The ribonuclease RNase J is a key enzyme in RNA turnover and precursor processing in the model Gram-positive bacterium Bacillus subtilis and numerous other bacterial and archaeal species (1–9). Thus, in addition to the eponymous β-lactamase fold, RNase J bears C-terminal and β-CASP domains. RNase J can cleave mRNA by either endonucleolytic or exonucleolytic mode, with preference depending on the 5′ end of the RNA.

The structure reveals a homotetrameric quaternary organization that unexpectedly carries intact nucleotides of RNA at each of the active sites. This pre-cleavage structure, solved at 2.27 Å resolution, provides details of the interactions of the RNA with the catalytic site, including a network of water molecules which may facilitate acid-base chemistry. In the course of preparing the recombinant S. coelicolor RNase J, RNA originating from the E. coli expression host was found to co-purify with the enzyme. The RNA was also sequenced and identified as 5′ pCGCCU, but the remaining 3′ nucleotides could not be identified unambiguously. The 5-nucleotide sequence fitted well into the experimental electron density in the substrate-binding tunnel that encompasses the active site, but the electron density was not clearly defined for the remaining nucleotides to the 3′ end of the experimentally identified pCGCCU sequence. The RNA interacts with both the metals through the O1 and O2 oxygens of the penultimate phosphate of the 5′ terminus. The water forms a close contact to the phosphate ester oxygen (2.7 Å). It was unexpected that the RNA would be found in the catalytic site adjacent to a water molecule that is apparently ‘activated’ by Zn binding, and yet not be cleaved. The reason that the S. coelicolor RNase J/RNA complex is stalled appears to be related to the presence of 1.33 mM EDTA in the crystallization condition, because we observe that EDTA inhibits the activity of the enzyme in this concentration range. Close inspection of the active site shows that the scissile phosphate is not properly aligned with the potentially attacking water molecule to permit a bimolecular nucleophilic (SN2) attack.

>MSHPHPELGRPPALPKGGLRVTPLGGLGEIGRNMTVFEYGGRLLIVDCGVLFPEEEQPGIDLILPDFTSIRDRLDDIEGIVLTHGHEDHIGGVPFLLREKPDIPLIGSKLTLALIEAKLQEHRIRPYTLEVAEGHRERVGPFDCEFVAVNHSIPDALAVAIRTPAGMVVHTGDFKMDQLPLDGRLTDLHAFARLSEEGIDLLLADSTNAEVPGFVPPERDISNVLRQVFANARKRIIVASFASHVHRIQQILDAAHEYGRRVAFVGRSMVRNMGIARDLGYLKVPPGLVVDVKTLDDLPDSEVVLVCTGSQGEPMAALSRMANRDHQIRIVNGDTVILASSLIPGNENAVYRVINGLTRWGANVVHKGNAKVHVSGHASAGELLYFYNICRPKNLMPVHGEWRHLRANAELGALTGVPHDRIVIAEDGVVVDLVEGKAKITGKVQAGYVYVDGLSVGDVGEPALKDRKILGDEGIISVFVVMDSSTGKITGGPHVQARGSGIEDSAFAAVLPKVTEALERSAQDGVVEPHQMQQLIRRTLGKWVSDTYRRRPMILPVVVEV[2x]>MKLKKIVFTLIALGLFSCKTTSVLVKNEPQLKTPKNVILLISDGAGLSQISSTFYFKSGTPNYTQFKNIGLIKTSSSREDVTDSASGATAFSCGIKTYNAAIGVADDSTAVKSIVEIAALNNIKTGVVATSSITEATPASFYAHALNRGLEEEIAMDMTESDLDFFAGGGLNYFTKRKDKKDVLAILKGNQFTINTTALTDFSSIASNRKMGFLLA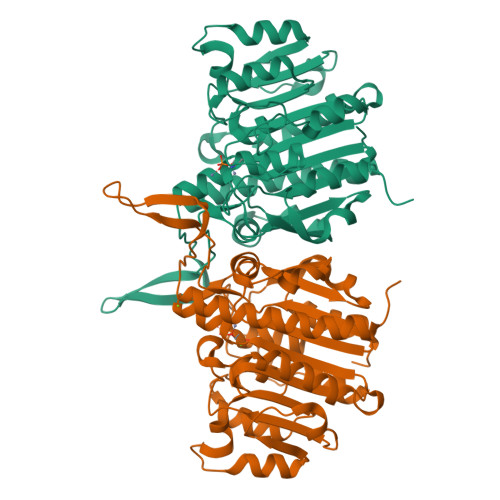DEAMPTMEKGRGNFLSAATDLAIQFLSKDNSAFFIMSEGSQIDWGGHANNASYLISEINDFDDAIGTALAFAKKDGNTLVIVTSDHETGGFTLAAKKNKREDGSEYSDYTEIGPTFSTGGHSATLIPVFAYGPGSEEFIGIYENNEIFHKILKVTKWNQ[2x]6,7-DINITROQUINOXALINE-2,3-DIONE 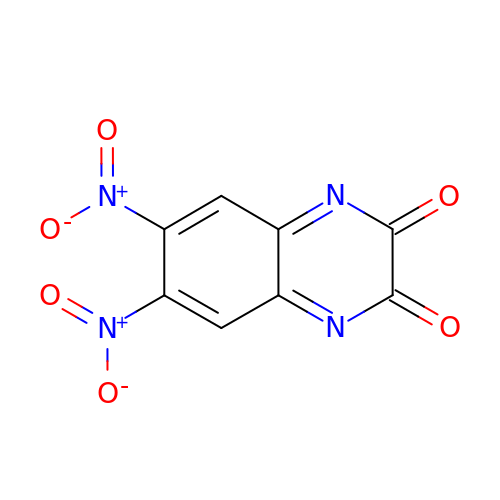| C8 H2 N4 O6 | YEUPBRRGMWBCEB-UHFFFAOYSA-N>KNVPSRAVKRVTAITKVEREAVLVCELPSFDVTDVEFDLFRARESTDKPLDVAAAIAYRLLLGSGLPQKFGCSDEVLLNFILQCRKKYRNVPYHNFYHVVDVCQTIHTFLYRGNVYEKLTELECFVLLITALVHDLDHMGLNNSFYLKTESPLGILSSASGNTSVLEVHHCNLAVEILSDPESDVFDGLEGAERTLAFRSMIDCVLATDMAKHGSALEAFLASAADQSSDEAAFHRMTME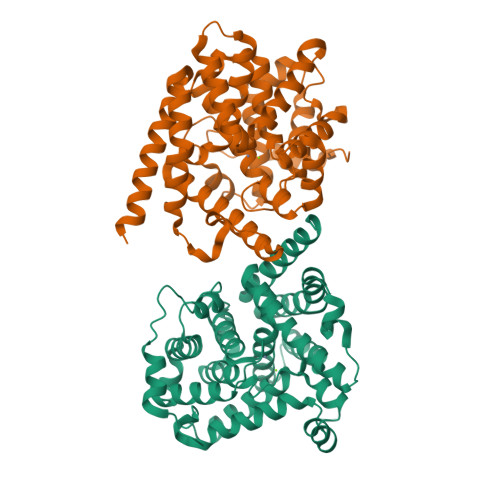IILKAGDISNVTKPFDISRQWAMAVTEEFYRQGDMEKERGVEVLPMFDRSKNMELAKGQIGFIDFVAAPFFQKIVDACLQGMQWTVDRIKSNRAQWERVLETR[2x]>GPLLAQSAKSMRTTEIETSGWEDALKWLRENTPEYSTATSWWDYGYWIESSLLGQRRASADGGHARDRDHILALFLARDGNISEVDFESWELNYFLVYLNDWAKFNAISYLGGAITRREYNGDESGRGAVTTLLPLPRYGEKYVNLYAKVIVDVSNSSVKVTVGDRECDPLMVTFTPSGKTIKGTGTCSDGNAFPYVLHLTPTIGVLAYYKVATANFIKLAFGVPASTIPGFSDKLFSNFEPVYESGNVIVYRFTPFGIYKIEENINGTWKQVYNLTPGKHELKLYISAFGRDIENATLYIYAINNEKIIEKIKIAEISHMDYLNEYPIAVNVTLPNATSYRFVLVQKGPIGVLLDAPKVNGEIRSPTNILREGESGEIELKVGVDKDYTADLYLRATFIYLVRKSGKDNEDYD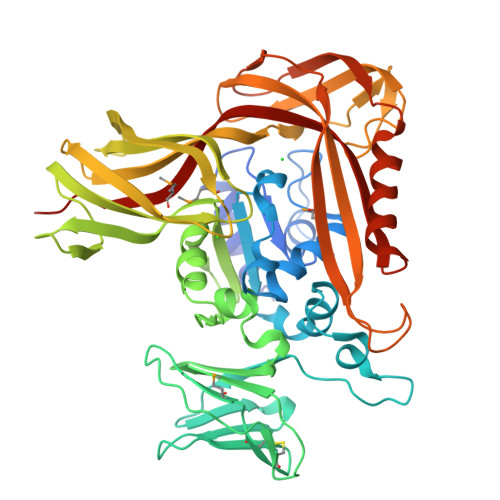AAFEPQMDVFFITKIGENIQLKEGENTVKVRAELPEGVISSYKDELQRKYGDKLIIRGIRVEPVFIAEKEYLMLEVSASAPHH[4x]>[2x]GMNTLLKQLKPYPFARLHEAMQGISAPEGMEAVPLHIGEPKHPTPKVITDALTASLHELEKYPLTAGLPELRQACANWLKRRYDGLTVDADNEILPVLGSREALFSFVQTVLNPVSDGIKPAIVSPNPFYQIYEGATLLGGGEIHFANCPAPSFNPDWRSISEEVWKRTKLVFVCSPNNPSGSVLDLDGWKEVFDLQDKYGFIIASD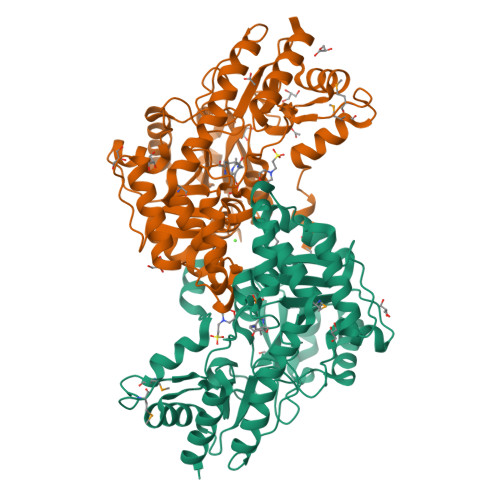ECYSEIYFDGNKPLGCLQAAAQLGRSRQKLLMFTSLSKRSNVPGLRSGFVAGDAELLKNFLLYRTYHGSAMSIPVQRASIAAWDDEQHVIDNRRLYQEKFERVIPILQQVFDVKLPDASFYIWLKVPDGDDLAFARNLWQKAAIQVLPGRFLARDTEQGNPGEGYVRIALVADVATCVKAAEDIVSLYR> GSHMATYYYALASQKFLLEEEPFEEVLKERRRDYGEKNKEIDFWQVIQPAFLNAPELAEAKAKAPEKNVAIVSTNKSFIVWVKLRLEYVLTGEFEAPSDAIPDPLASLD

Mg-protoporphyrin IX monomethylester cyclase (MgPME–cyclase) catalyses the formation of the isocyclic E ring by cyclising the methyl propionate side-chain at C-13 to the C-15 bridge carbon between rings C and D, generating protochlorophyllide (Pchlide). Recently, the small monomeric protein Ycf54 was identified as a second candidate component of the MgPME–cyclase. The Ycf54 protein has been identified as a component of the MgPME–cyclase complex.

We crystallised the WT Ycf54 protein and solved the structure using molecular replacement to a resolution of 1.3 Å. Synechocystis Ycf54 is composed of a single domain (annotated as the Ycf54 domain in PFAM), in which a central four-stranded antiparallel β-sheet (β1–β4) is flanked on one side by helices α1, α2 and α5 and by helices α3 and α4 on the other. This domain appears to be typical of the Ycf54 superfamily, with Synechocystis Ycf54 representing the most complete and highest resolution structure to date. An additional conserved structural feature is an electronegative ridge that extends across one face of the protein. This ridge is located on α2 of Synechocystis Ycf54, where two of the highly conserved residues, E22 and E26, contribute to its negative charge. Although individually point mutating these residues to alanine yielded no discernible phenotype, the fact that the ridge is unusual and structurally conserved indicates that it may be of physiological importance. In WT Ycf54, R82 adopts two clearly defined conformations, both of which form stabilising hydrogen bonds with neighbouring residues. In one conformation, R82 forms a water-mediated hydrogen bond with the side chain of W78, and in the other R82 forms two direct hydrogen bonds with the backbone carbonyl of F20 and the side chain of E17. On the WT Ycf54 structure, residues D39A and F40A are not particularly surface exposed, so we are unable to speculate as to how these mutations result in a reduced interaction with CycI.> GSHMLRLSAPGQLDDDLCLLGDVQVPVFLLRLGEASWALVEGGISRDAELVWADLCRWVADPSQVHYWLITHKHYDHCGLLPYLCPRLPNVQVLASERTCQAWKSESAVRVVERLNRQLLRAEQRLPEACAWDALPVRAVADGEWLELGPRHRLQVIEAHGHSDDHVVFYDVRRRRLFCGDALGWFDEAE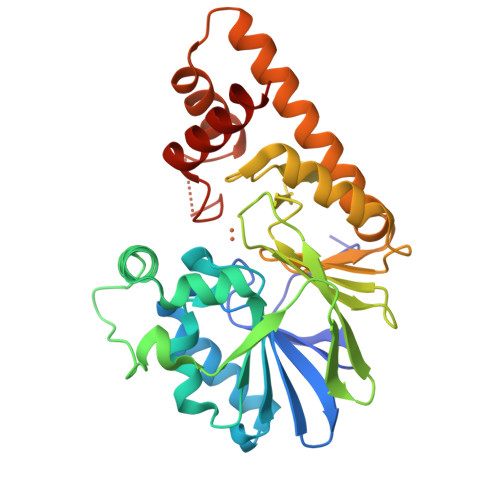GVWRPLVFDDMEAYLESLERLQRLPTLLQLIPGHGGLLRGRLAADGAESAYTECLRLCRRLLWRQSMGESLDELSEELHRAWGGQSVDFLPGELHLGSMRRMLEILSRQALPLD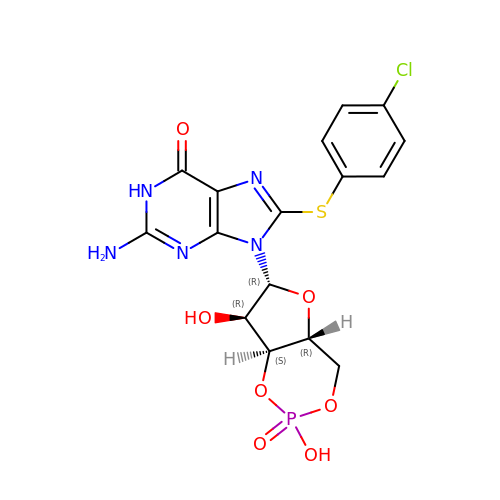2-(~2~H_2_)amino-8-[(4-chlorophenyl)sulfanyl]-9-[(2S,4aR,6R,7R,7aS)-2-hydroxy-7-(~2~H)hydroxy-2-oxotetrahydro-2H,4H-2lambda~5~-furo[3,2-d][1,3,2]dioxaphosphinin-6-yl](~2~H)-1,9-dihydro-6H-purin-6-one | C16 H15 Cl N5 O7 P S | ZDJHIEHUVPCEDK-IDTAVKCVSA-N> GTLRFFTVTDEYIAYLRKFESKVHYQYENNASTYVGVVLKKNDFNYFIPLLSYKKGNPEKDKAMKKRSRIVTRLFEIGNINNPLGYLLHHNMIPVPDSELI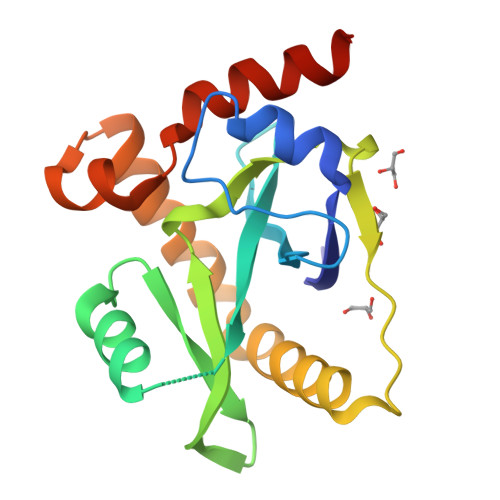PLPLDLKKPKHKMMQKQLIYMKSISEKIENKSEVVYRKAAHEKDGYYLKFSCDFKLLEAKATLYSKKSTFQ> MKLYFNGGKKKKIRAVDFVGTIAKIDGVSADDIGIITIMDNASYVEILNGKGPHVLKVMKNTTVK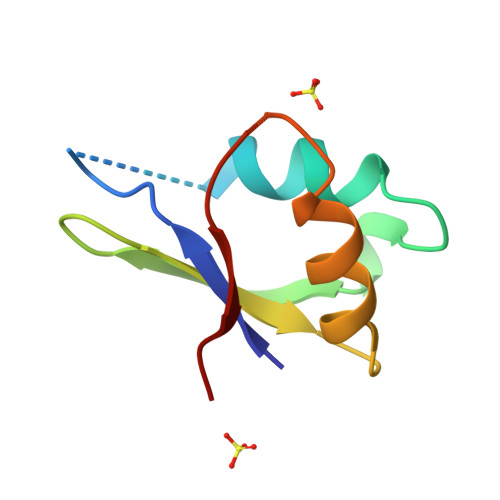GKQLKVNKANK>[2x]GSMAPLVKNEPQH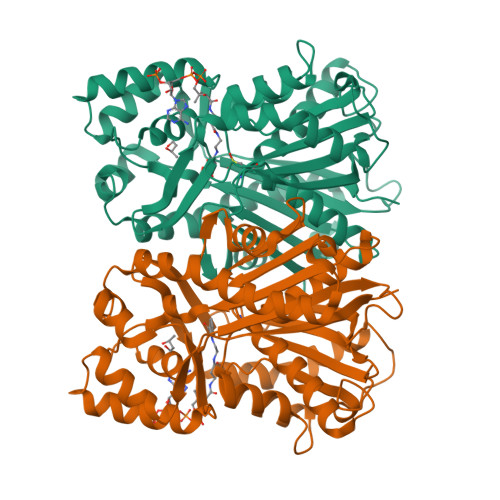AKILAIGTANPPNVYHQKDYPDFLFRVTKNEHRTDLREKFDRICEKSRTKKRYLHLTEEMLKANPNIYTYGAPSLDVRQDICNIEVPKLGQEAALKAIKEWGQPISRITHLIFCTASCVDMPGCDFQLIKLLGLDPSVTRTMIYEAGCYAGATVLRMAKDFAENNKGARVLVVCAEITTVFFHGLTDTHLDILVGQALFADGASAVIVGANPEPEIERPLFEIVACRQTILPNSEHGVVVNIREMGFNYYLSGDVPKFVGGNVVDFMTKTFEKVDGKKKDWNSLFFSVHPGGPAIVDQVEEKLGLKEGKLRATRHVLSEYGNMGAPTVHFILDEMRNKSIEEGKTTTGEGLEWGVVIGIGPGLTVETAVLRSESIRC> MKELNDLEKKYNAHIGVYALDTKSGKEVKFNSDKRFAYASTSHAINSAILLEQVPYNKLNKKVHINKDDIVAYSPILEKYVGKDITLKALIEASMTYSDNTANNKIIKEIGGIKKVKQRLKELGDKVTNPVRYEIELNYYSPKSKKDTSTPAAFGKTLNKLIANGKLSKENKKFLLDLMLNNKSGDTLIKDGVPKDYKVADKSGQAITYASRNDVAFVYPKGQSEPIVLVIFTNK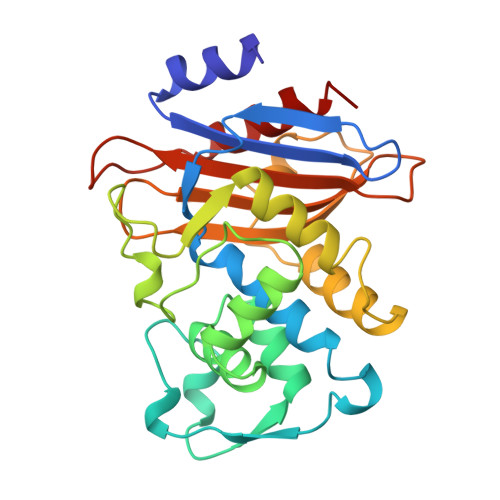DNKSDKPNDKLISETAKSVMKEF>[2x]SNYLDQMEEYDKV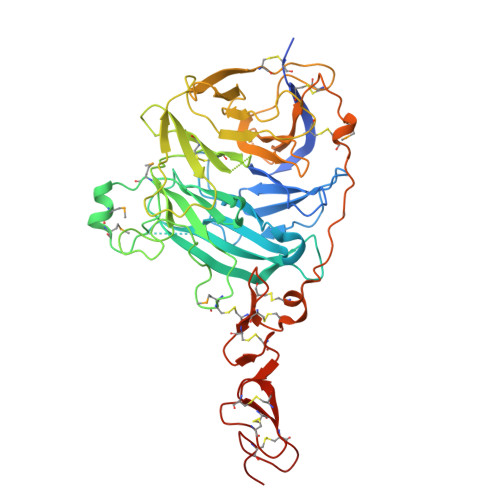EEISRKHKHNCFCIQEVVSGLRQPVGALHSGDGSQRLFILEKEGYVKILTPEGEIFKEPYLDIHKLVQSGIKGGDERGLLSLAFHPNYKKNGKLYVSYTTNQERWAIGPHDHILRVVEYTVSRKNPHQVDLRTARVFLEVAELHRKHLGGQLLFGPDGFLYIILGDGMITLDDMEEMDGLSDFTGSVLRLDVDTDMCNVPYSIPRSNPHFNSTNQPPEVFAHGLHDPGRCAVDRHPTDININLTILCSDSNGKNRSSARILQIIKGKDYESEPSLLEFKPFSNGPLVGGFVYRGCQSERLYGSYVFGDRNGNFLTLQQSPVTKQWQEKPLCLGTSGSCRGYFSGHILGFGEDELGEVYILSSSKSMTQTHNGKLYKIVDPKRPLMPEECRATVQPAQTLTSECSRLCRNGYCTPTGKCCCSPGWEGDFCRTAKCEPACRHGGVCVRPNKCLCKKGYLGPQCEHHHHHH>GUAUGUAC[2x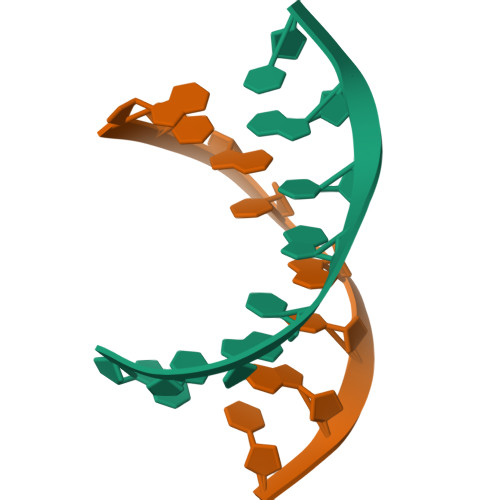]> RALAAPLVHHHHHHALDENLYFQGALADVSRPPHARKTGGSSPETKYDQPPKCDISGKEAIS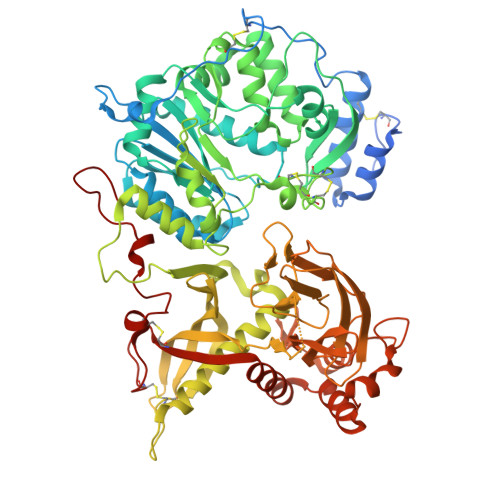ALSRAKSKHCRQEIGETYCRHKLGLLMPEKVTRFCPLEGKANKNVQWDEDSVEYMPANPVRIAFVLVVHGRASRQLQRMFKAIYHKDHFYYIHVDKRSNYLHRQVLQVSRQYSNVRVTPWRMATIWGGASLLSTYLQSMRDLLEMTDWPWDFFINLSAADYPIRTNDQLVAFLSRYRDMNFLKSHGRDNARFIRKQGLDRLFLECDAHMWRLGDRRIPEGIAVDGGSDWFLLNRRFVEYVTFSTDDLVTKMKQFYSYTLLPAESFFHTVLENSPHCDTMVDNNLRITNWNRKLGCKCQYKHIVDWCGCSPNDFKPQDFHRFQQTARPTFFARKFEAVVNQEIIGQLDYYLYGNYPAGTPGLRSYWENVYDEPDGIHSLSDVTLTLYHSFARLGLRRAETSLHTDGENSCRYYPMGHPASVHLYFLADRFQGFLIKHHATNLAVSKLETLETWVMPKKVFKIASPPSDFGRLQFSEVGTDWDAKERLFRNFGGLLGPMDEPVGMQKWGKGPNVTVTVIWVDPVNVIAATYDILIESTAEFTHYKPPLNLPLRPGVWTVKILHHWVPVAETKFLVAPLTFSNRQPIKPEEALKLHNGPLRNAYMEQSFQSLNPVLSLPINPAQVEQARRNAASTGTALEGWLDSLVGGMWTAMDICATGPTACPVMQTCSQTAWSSFSPDPKSELGAVKPDGRLR> MLHGTPVRRASLRYRRPYWMMFLKGVDNWKIYTVIQQPDHQRTEMLYQAWLGGLDRPYTRPKCMANQPLWLSKKRHMLRKERLDGPETPLEKYVLEWHKKFHSFQGTERPTPDDLHTALDLVERPLDLSYALQLLGQCRNLNNIRFAKETFL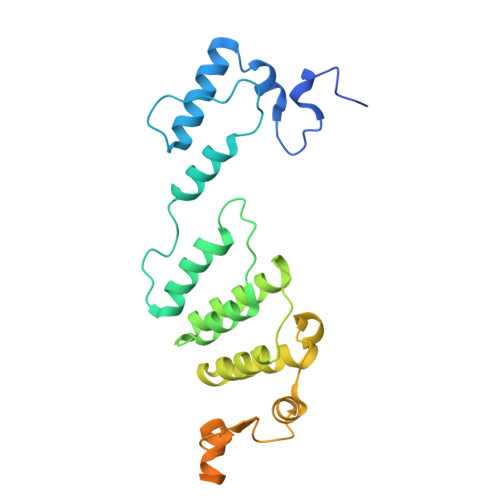VFLEACLRVGRRDCAEYALEHAEPLGFWFIDEDHRRYLQGEQTWYKLSPLDNLYYPVEENAKLNEGRKPITRLSPATESPGSGTAISDGEPSTDVEGETTVDDEIAQLEAELAALEREGGGK>MSAKAISEQTGKELLYKFICTTSAIQNRFKYARVTPDTDWARLLQDHPWLLSQNLVVKPDQLIKRRGKLGLVGVNLTLDGVKSWLKPRLGQEATVGKATGFLKNFLIEPFVPHSQAEEFYVCIYATREGDYVLFHHEGGVDVGDVDAKAQKLLVGVDEKLNPEDIKKHLLVHAPEDKKEILASFISGLFNFYEDLYFTYLEINPLVVTKDGVYVLDLAAKVDATADYICKVKWGDIEFPPPFGREAYPEEAYIADLDAKSGASLKLTLLNPKGRIWTMVAGGGASVVYSDTICDLGGVNELANYGEYSGAPSEQQTYDYAKTILSLMTREKHPDGKILIIGGSIANFTNVAATFKGIVRAIRDYQGPLKEHEVTIFVRRGGPNYQEGLRVMGEVGKTTGIPIHVFGTETHMTAIVGMALGHRPIPMGKSTTLFSRHTKAIVWGMQTRAVQGMLDFDYVCSRDEPSVAAMVYPFTGDHKQKFYWGHKEILIPVFKNMADAMRKHPEVDVLINFASLRSAYDSTMETMNYAQIRTIAIIAEGIPEALTRKLIKKADQKGVTIIGPATVGGIKPGCFKIGNTGGMLDNILASKLYRPGSVAYVSRSGG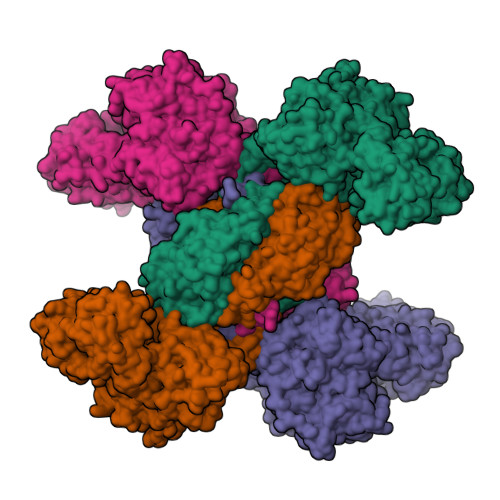MSNELNNIISRTTDGVYEGVAIGGDRYPGSTFMDHVLRYQDTPGVKMIVVLGEIGGTEEYKICRGIKEGRLTKPIVCWCIGTCATMFSSEVQFGHAGACANQASETAVAKNQALKEAGVFVPRSFDELGEIIQSVYEDLVANGVIVPAQEVPPPTVPMDYSWARELGLIRKPASFMTSICDERGQELIYAGMPITEVFKEEMGIGGVLGLLWFQKRLPKYSCQFIEMCLMVTADHGPAVSGAHNTIICARAGKDLVSSLTSGLLTIGDRFGGALDAAAKMFSKAFDSGIIPMEFVNKMKKEGKLIMGIGHRVKSINNPDMRVQILKDYVRQHFPATPLLDYALEVEKITTSKKPNLILNVDGLIGVAFVDMLRNCGSFTREEADEYIDIGALNGIFVLGRSMGFIGHYLDQKRLKQGLYRHPWDDISYVLPEHMSMGGSHHHHHH[8x]>MVLNSNELEHIHSTNHSVNDISIRWGVIGAGQKGNKEADLFAGYKFSNGTTCYPTLAVNFAESDMMHLQNIIKEDRIHFDGLKGAARTPSVVTDLFDPETNPNANGYLDKLAQELGRKFTNEEGEVIVDQFLICLGAGGGVGTGWGSLVLQLIREQFFPCPVSMLISLPSGDPDEINNALVLLSEIDEFMREQDRLFGNSDIKPLANVIVNDNTQMQRIIESQKGTKDLKNRYVNWKEVANDNVVSTLHEINIIPENYGSDNVTYDPSDLIKLLSIPGRFLTIGKARIAKFDLHSLENSIKRSLDEGFFSAEHQFETATMYGGFVLRPSNADFFKDVNTENRIRNTLGEYKRLDEIAGKFGDPIWDNEYAVCYTIFAGMTMPKRYISLAREGKELAEKQEQLRAEAQRKQDEEKV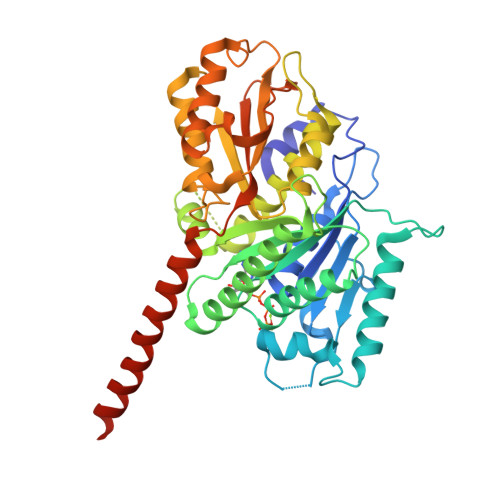DISFAT[7x]> KNTASRSAASVPANEQISQLASLVAA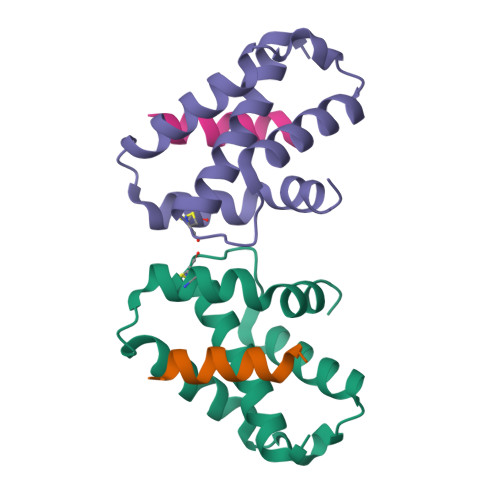SKYLRVQCERSDLPDDGTILKTAVNVAVQKGWDTGRYQSLPQLSENLYQGLLKDGTPKATQCSSFNRTMTPFLDAMRTVR;> RTFRQVQSSISDFYD> LRSRRVDVMDVMNRLILAMDLMNRDDALRVTGEVREYIDTVKIGYPLVLSEGMDIIAEFRKRFGCRIIADFKVADIPETNEKICRATFKAGADAIIVHGFPGADSVRACLNVAEEMGREVFLLTEMSHPGAE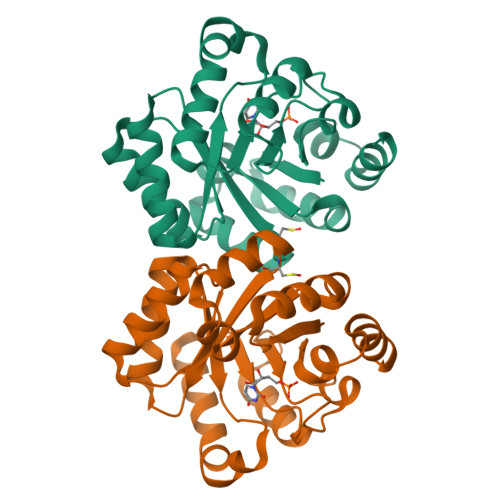MFIQGAADEIARMGVDLGVKNYVGPSTRPERLSRLREIIGQDSFLISPGVGAQGGDPGETLRFADAIIVGRSIYLADNPAAAAAGIIESIKDLLNP>MGAQVSTQKTGAHETGLNASGNSIIHYTNMNYYKDSASNSANRQEFAQDPGKFTEPVKDIMIKSMPALNSPSAEECGYSDRVRSITLGNSTITTQECANVVVGYGTWPTYLRDEEATAEDQPTQPDVATCRFYTLESVMWQQSSPGWWWKFPDALSNMGLFGQNMQYHYLGRAGYTLHVQCNASKFHQGCLLVVCVPEAEMGCATIANKPDQKSLSNGETANVFDSQNTSGQTAVQANVINAGMGIGVGNLTIFPHQWINLRTNNSATIVMPYVNSVPMDNMFRHNNFTLMIIPFAPLSYSTGATTYVPITVTVAPMCAEYNGLRLAGRQGLPTMLTPGSNQFLTSDDFQSPSAMPQFDVTPEMAIPGQVNNLMEIAEVDSVVPVNNTEGKVMSIEAYQIPVQSNSTNGSQVFGFPLIPGASSVLNRTLLGEILNYYTHWSGSIKLTFMFCGSAMATGKFLLAYSPPGAGAPTTRKEAMLGTHVIWDVGLQSSCVLCIPWISQTHYRYVVMDEYTAGGYITCWYQTNIVVPADTQSDCKILCFVSACNDFSVRMLKDTPFIKQDSFFQGPPGEAIERAIARVADTISSGPVNSESIPALTAAETGHTSQVVPADTMQTRHVKNYHSRSESTVENFLCRSACVYYTTYKNHGTDGDNFAQWVINTRQVAQLRRKLEMFTYARFDLELTFVITSSQEQSTIKGQDSPVLTHQIMYVPPGGPVPTKINSYSWQTSTNPSVFWTEGSAPPRISIPFISIGNAYSMFYDGWARFDKQGTYGINTLNNMGTLYMRHVNDGSPGPIVSTVRIYFKPKHVKTWVPRPPRLCQYQKAGNVNFEPSGVTEGRTEITAMQTT[4x]

Enteroviruses are nonenveloped positive single-stranded (ss) RNA viruses and are major causative agents of waterborne diseases. Coxsackievirus B5 (CVB5) is a genotype of the Enterovirus genus, which is frequently detected in clinical and wastewater surveillance. Here, we employed a reverse genetic system for CVB5 and assessed how different amino acid substitutions in capsid proteins affects the virus’ sensitivity to free chlorine and heat. To elucidate the mechanism behind reduced heat sensitivity of the CVB5F.cas.genogroupB mutant, we subjected it to analysis by cryoEM.

We applied a combination of 2D and 3D classification steps in cryoSPARC package to separate the particles corresponding to mature virions (F), intermediate-altered state (A), and empty viral capsids (E). The resulting EM density maps were at 3.6, 2.7, and 2.6 Å global resolution for the capsid-corresponding part of particles F, A, and E, respectively, thus allowing building of atomic models of each state. Surprisingly, only ∼0.2% of the total data set corresponded to mature virions in the F state (193 particles). We believe this to be a result of formaldehyde inactivation. Nevertheless, the reconstructed atomic model closely matched the previously published CVB5 structure based on genogroup A (and a previous study64). The root-mean-square deviation (RMSD) of Cα positions between the two structures was 0.45 Å. This is consistent with the fact that most mutations were relatively conservative (L → I, E → D, S → T, K → R) and unlikely to induce major structural rearrangements. None of the mutations were located at the interfaces of multiple protomers (each comprising a single copy of VP1–4). Amino acids at this position make direct contact with the noncovalently bound palmitate residue (i.e., the pocket factor). While we noticed somewhat weaker density for the pocket factor compared to the previously published cryoEM map of CVB5 F-particle (EMD-3032164), the switch from M to I does not alter the size of the hydrophobic pocket, and these two amino acids are commonly found at position 180 across the Enterovirus genus relevant to human infection, including 112 exemplar strains of each genotype of Enterovirus A, B, C, and D, listed in Virus Metadata Resource.>[3x]MNRLPYFINYFFDTYLLISEDTPVGSSVTQLLARDMDNDPLVFGVSGEEASRFFAVESETGVVWLRQPLDRETKSEFT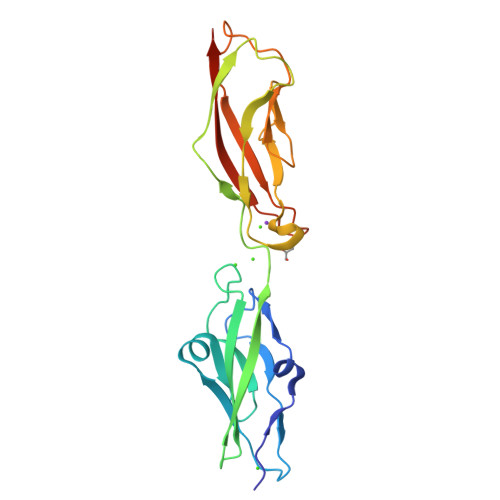VEFSVSDSQGVITRKVNIQVGDVNDNAPRFHNQPYSVRIPENTPVGTPIFIVNATDPDLGAGGSVLYSFQPPSHFFAIDSGRGIVTVIRELDYEVTQAYQLQVNATDQDKTKPLSTLANLAITITDLEHHHHHH> GRPEWIWLALGTALMGLGTLYFLVKGMGVSDPDAKKFYAITTLVPAIAFTMYLSMLLGYGLTMVPFGGEQNPIYWARYADWLFTTPLLLLDLALLVDADQGTILALVGADGIMIGTGLVGALTKVYSYRFVWWAISTAAMLYILYVLFFGFTSKAESMRPEVASTFKVLRNV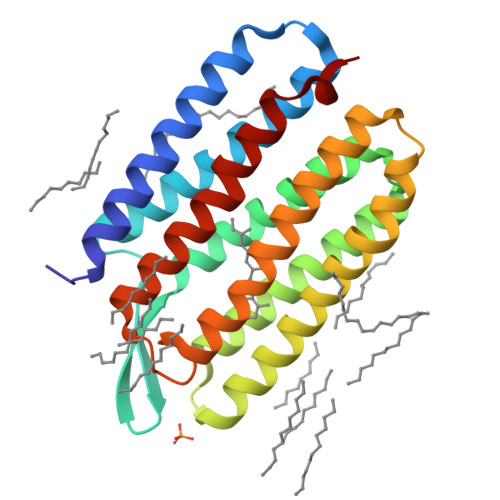TVVLWSAYPVVWLIGSEGAGIVPLNIETLLFMVLDVSAKVGFGLILLRSRAIFG4,6-difluoro-1,3-benzothiazol-2-amine | C7 H4 F2 N2 S | 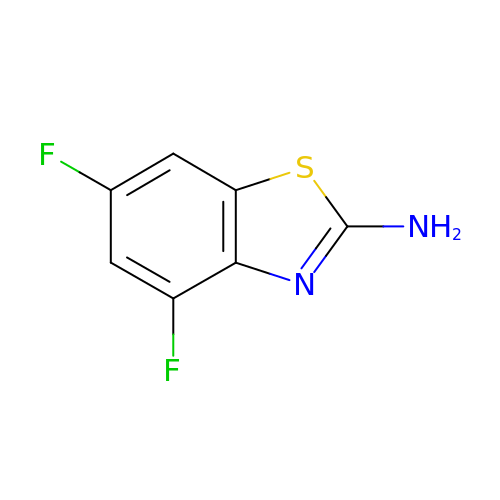DDKKXSCVPKDRRS-UHFFFAOYSA-N N-{6-[(2S)-2-methylpyrrolidin-1-yl]pyridin-2-yl}-6-phenylimidazo[1,2-b]pyridazin-8-amine | C22 H22 N6 | 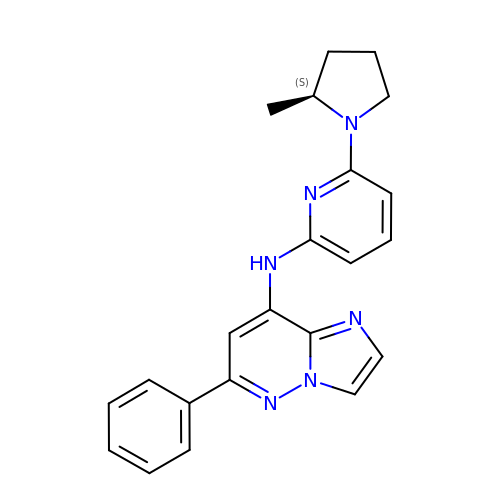OLNOLIZABHZSEW-INIZCTEOSA-N> MLHGSLPSLASLRYRRPYWMLFLKDVDNWKIYTVIQQPDHQRTEMLYQAWLGGLDRPYTRPKCMANQPLWLSKKRHILRKDRLDGPETPLEKYVLEWHKRFHSFQGTERPTVDDLHTALDLVERPLDLSYAFQLLNQCRNVNNIRFAKDTFLVFLEACLRVDRKDCALYATENAEALGFWHIEEDYRRYLRGEQSWYRLSPLDNMYYPLEENVKLNAGRSPPSSAAVAEGDAEGTAETTGFEAAAGAAAWSDDEGS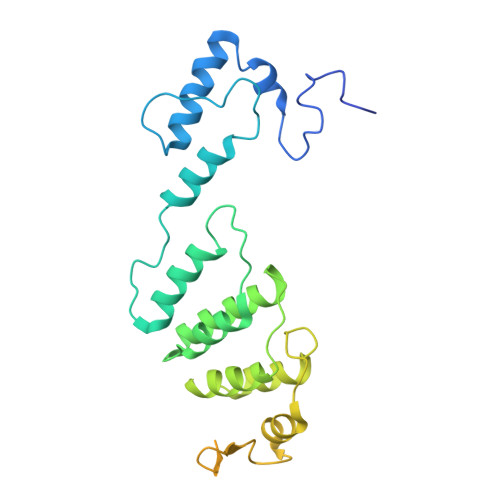MKAGSSRESMTVDDEIARLEAELAALEEEGTDGDNDVKGPKGH> GPPGPPGPPGPPGPRGRTGPPG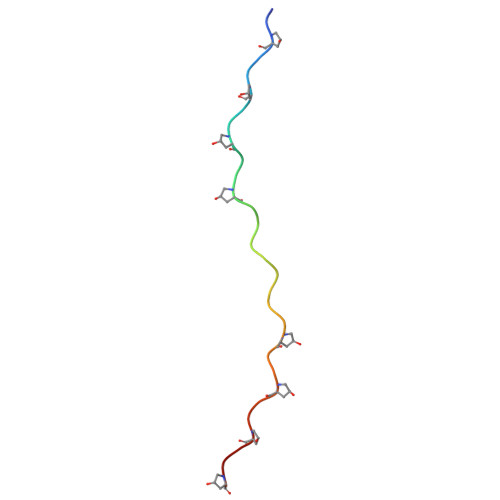PPGPPGPP5-BROMO-9-AMINO-N-ETHYL(DIAMINOMETHYL)ACRIDINE-4-CARBOXAMIDE 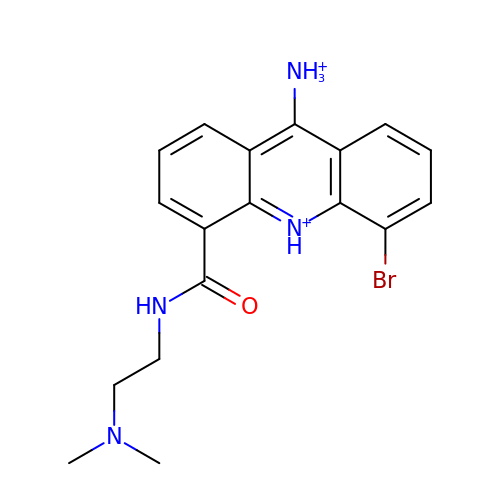| C18 H21 Br N4 O | NROQPXQSDDINMC-UHFFFAOYSA-P> MVYRRRRGRGRRARPMSSLGRLLYRKPWLMHPRFRARYRWRRKNGITNLRLTRQVELWVPKDAANASFYVNHYTFDLDDFIPAGTQLNSSPLPFKYYRIRKVKVEFQPRLPITSPFRGYGSTVPILDGAFVTPATGESDPIWDPYINFSGRHVIRTPAWYHKRYFTPKPLIDGNTGFFQPNNKQNALWFPNKQGQNIQWSGLGFAMQKGNEAYNYQ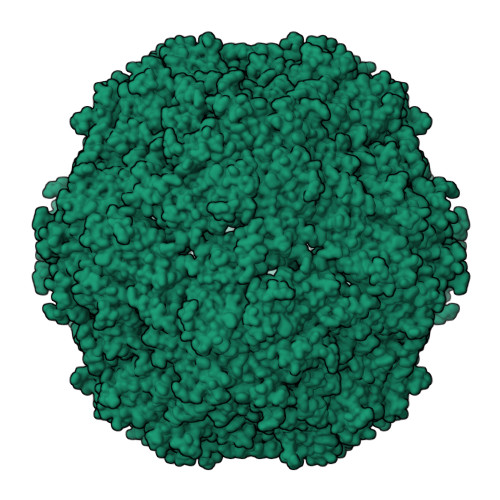VRFTLYVQFREFDLFNN>MKMDYKEQSHIIPTYKRFDIVLEKGQGVYLFDDKAKKYLDFSSGIGVCALGYNHAKFNAKIKAQVDKLLHTSNLYYNENIAAAAKNLAKASALERVFFTNSGTESIEGAMKTARKYAFNKGVKGGQFIAFKHSFHGRTLGALSLTANEKYQKPFKPLISGVKFAKYNDISSVEKLVNEKTCAIILESVQGEGGINPANKDFYKALRKLCDEKDILLIADEIQCGMGRSGKFFAYEHAQILPDIMTSAKALGCGLSVGAFVINQKVASNSLEAGDHGSTYGGNPLVCAGVNAVFE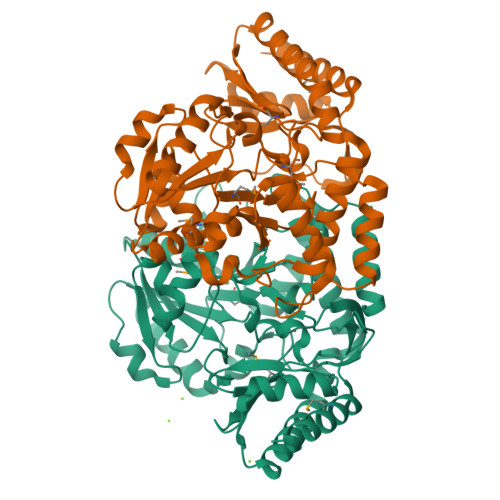IFKEEKILENVNKLTPYLEQSLDELINEFDFCKKRKGLGFMQGLSLDKSVKVAKVIQKCQENALLLISCGENDLRFLPPLILQKEHIDEMSEKLRKALKSF[2x]> MHHHHHHHHHHQRGPGFKFVDLNEKELQNEIKQLGSDSSDGHNSEKKDTDGADENVQIGEDFMEVDYEDKDNPVDSRNETDHKTNENGETDDNIETVMTQEQFVKRRRDMLEHINLAMNESSLALEFVSLLLSSVK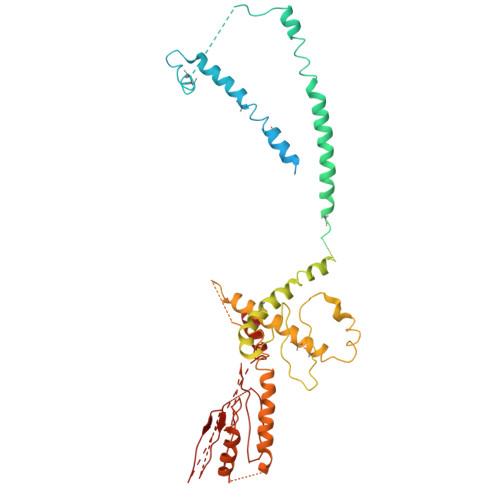ESTGMSSMSPFLRKVVKPSSLNSDKIPYVAPTKKEYIELDILNKGWKLQSLNESKDLLRASFNKLSSILQNEHDYWNKIMQSISNKDVIFKIRDRTSGQKLLAIKYGYEDSGSTYKHDRGIANIRNNIESQNLDLIPHSSSVFKGTDFVHSVKKFLRVRIFTKIESEDDYILSGESVMDRDSESEEAETKDIRKQIQLLKKIIFEKELMYQIKKECALLISYGVSIENENKVIIELPNEKFEIELLSLDDDSIVNHEQDLPKINDKRANLMLVMLRLLLVVIFKKTLRSRISSPHGLINLNVDDDILIIRPILGKVRFANYKLLLKKIIKDYVLDIVPGSSITETEVEREQPQENKNIDDENITKLNKEIRAFDKLLNIPRREXXXXXXXXXXXXXXXXXXXXXXXXXXXXXXXXXXXXXXXXXXXXXEVEDFLHFIVAEYIQQKKV The heterologous expression of the POD genes from the P. ostreatus genome, and subsequent kinetic studies, reveal a peroxidase array consisting of three VPs and six MnPs. The VP1 and MnP4 crystal structures were solved as representative for the two POD families present in the P. ostreatus genome. The overall structure of VP1 and MnP4 showed a heme group dividing the protein into a distal largely helical domain (formed by four main helices and two to three small ones) with one structural calcium ion, and a proximal domain composed by another six helices and a non-ordered region stabilized by a second calcium ion. The site where this takes place is conserved and comprises three acidic residues (E36/E40/D175 in VP1 and E36/E40/D181 in MnP4) located near the heme propionate occupying the most internal position with respect to the main access channel.

Concerning short MnP, whose crystal structure is now solved for the first time (from P. ostreatus MnP4), its main structural difference from P. chrysosporium long MnP concerns the existence of a more exposed Mn oxidation site, due to the absence of the C-terminal extension that in P. chrysosporium MnP (with a total of 357 residues) is partially fixed by a fifth disulfide bridge. The oxidation of lignin-related substrates was not detected in MnP4, where the active tryptophan is substituted by an alanine (left). The ability to oxidize Mn2+ completely disappeared after the simple E36A, E40A, or D179A mutations in MnP4, and also after the double E35A/E39A mutation in VP1 (the simple E35A, E39A, and D175A VP1 variants lost over 99.8% of their catalytic efficiency but retained detectable activity on Mn2+). At this site, the P56 to G59 loop of VP1 presents a six-residue insertion in MnP4 forming a small extra helix that protrudes into the solvent. Also, residues A130 and V131 in this VP1 region adopted a different conformation with respect to V135 and T136 in MnP4. These changes allow the F62 hydrophobic side chain of MnP4 to interact with K137 and, due to this interaction, the hydroxyl group of T136 interacts with one of the waters coordinating the distal calcium ion. Most of them involve the change of small hydrophobic side chains in VP1 for large hydrophilic side chains, such as the substitution of G290 in VP1 by K296 in MnP4. This lysine has interactions with D198 and D200, which are directly involved in the coordination of the proximal calcium. When the MnP4 crystal structure was solved, a striking observation was the high number of solvent-exposed lysines (a total of 20) and other basic residues (up to a total of 34). Another noteworthy characteristic of MnP4 is the high number of surface-exposed lysines (up to a total of 20) and other alkaline residues (up to a total of 35) compared with the other P. ostreatus PODs, which would result in a higher net positive charge of the protein and increased stability at acidic pH.

> MAKCSKGRTASNDACCVWFDVLDDIQENLFDGGECGEEVHESLRLTFHDAIGFSPALTRQGKFGGGGADGSIMLFSDIETNFAANNGVDDIVEQQKPIAIKHQVSFGDFIQFAGAVGSSNCAGGPRIQFLAGRSNVTKPSPDHLVPEPFDSVTSILARMGDAGFKPDEVVALLASHSVAAQDTIDPKLAGHPFDSTPSDFDSQFFVETLLKGTLIPGDSLHKGQVKSPLPGEFRLQSDELLARDSRTSCEWQSFISNPNSMVPKFERAMAKMATLGQNPKKLIDCSEVIPVPRGRVKQPTLPAGKTIKDIEASCRKAPFPRLPTDKGTFTSILPVPSS> HSQGTFTSDYSKYLDSKKAQEFV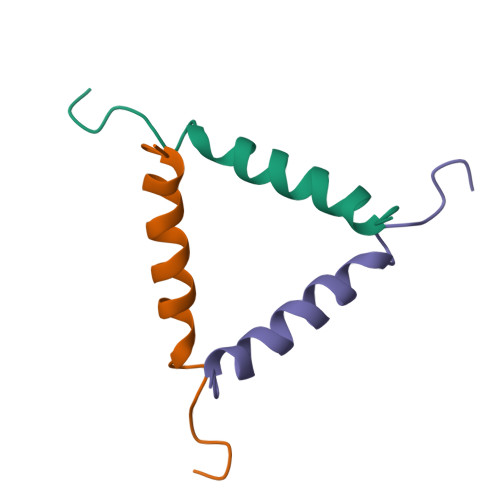QWLMNT> RSPWLGTLPAFLPCELKPHGLVDCNWLFLKSVPRFSAAASCSNITRLSLISNRIHHLHNSDFVHLSNLRQLNLKWNCPPTGLSPLHFSCHMTIEPRTFLAMRTLEELNLSYNGITTVPRLPSSLVNLSLSHTNILVLDANSLAGLYSLRVLFMDGNCYYKNPCTGAVKVTPGALLGLSQLTHLSLKYNNLTKVPRQLPPSLEYLLVSYNLIVKLGPEDLAQLTSLRVLDVGGNCRRCDHAPNPCIECGQKSLHLHPETFHHLSHLEGLVLKDSSLHTLNSSWFQGLVQLSVLDLSENFLYESITHTNAFQNLTRLRKLNLSFNYRKKVSFARLHLASSFKNLVSLQELNMNGIFFRLLNKYTLRWLADLPKLHTLHLQMNFINQAQLSIFGTFRALRFVDLSDNRISGPSTLSEATPEEADDAEQEELLSADPHPAPLSTPASKNFMDRCKNFKFTMDLSRNNLVTIKPEMFVQLSRLQCLSLSHNSIAQAVNGSQFLPLTNLQVL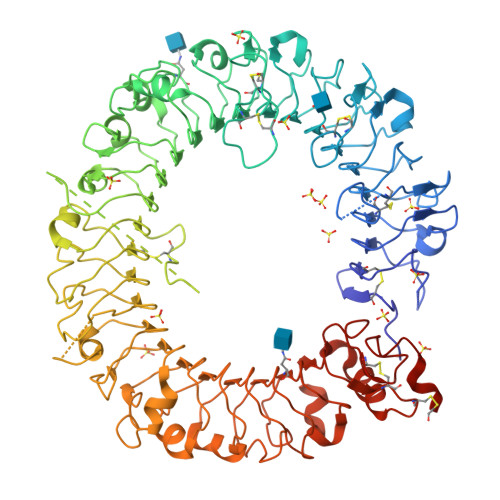DLSHNKLDLYHWKSFSELPQLQALDLSYNSQPFSMKGIGHQFSFVTHLSMLQSLSLAHNDIHTRVSSHLNSNSVRFLDFSGNGMGRMWDEGGLYLHFFQGLSGLLKLDLSQNNLHILRPQNLDNLPKSLKLLSLRDNYLSFFNWTSLSFLPNLEVLDLAGNQLKALTQGTLPNGTLLQKLDVSSNSIVSVVPAFFALAVELKEVNLSHNILKTVDRSWFGPIVMQLTVLDVRSNPLHCACGAAFVDLLLEVQTKVPGLANGVKCGSPGQLQGRSIFAQDLRLCLDEVLSWDEFLVPR2-[[(3~{S})-2,5-bis(oxidanylidene)pyrrolidin-3-yl]carbamoyl]-6-nitro-benzoic 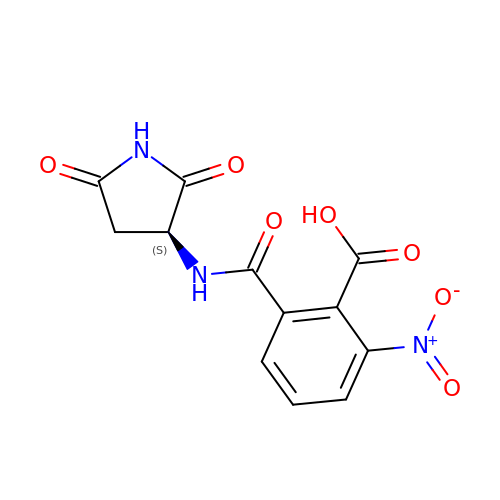acid | C12 H9 N3 O7 | DWGKCZUFQWKKEW-LURJTMIESA-N> MANPYERGPDPTESSIEAVRGPFAVAQTTVSRLQADGFGGGTIYYPTDTSQGTFGAVAISPGFTAGQESIAWLGPRIASQGFVVITIDTITRLDQPDS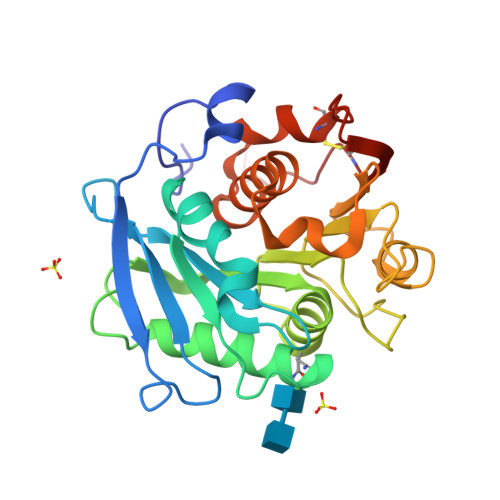RGRQLQAALDHLRTNSVVRNRIDPNRMAVMGHSMGGGGALSAAANNTSLEAAIPLQGWHTRKNWSSVRTPTLVVGAELDTIAPVSSHSEAFYNSLPSDLDKAYMELRGASHTVSNTPDTTTAKYSIAWLKRFVDKDLRYEQFLCPAPDDFAISEYRSTCPFHHHHHH> MAKEKARYFTFLLYPESIPSDWELKLETLG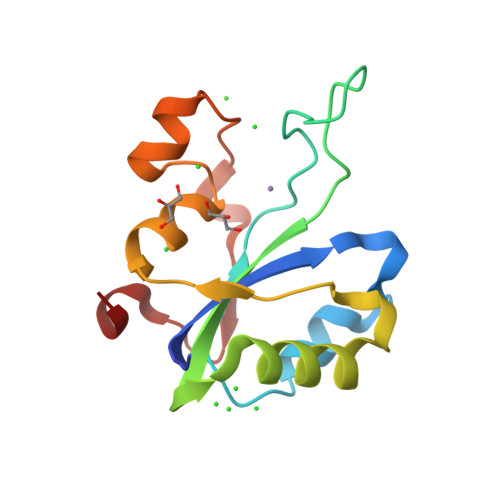VPMAISPLHDKDKSSIKGQKYKKAHYHVLYIAKNPVTADSVRKKIKLLLGEKSLAMVQVVLNVENMYLYLTHESKDAIAKKKHVYDKADIKLINNFDIDRYV>MSSTKQITLYTATFSPYAHRVRIALEEAGAEYTTYDVDILRNMPDWFPLVNPLKKIPAMTFGGPEVPPDQPSPESAKIAESLAMLEFIADLFPDAKLLPTDPVLRARARTFMALYENYVNGQFRDVWFLGTPADPLLQALEMLQGALPPDGGFAAGEWSIADAAVIPFLARMFPYLEAGLGLYS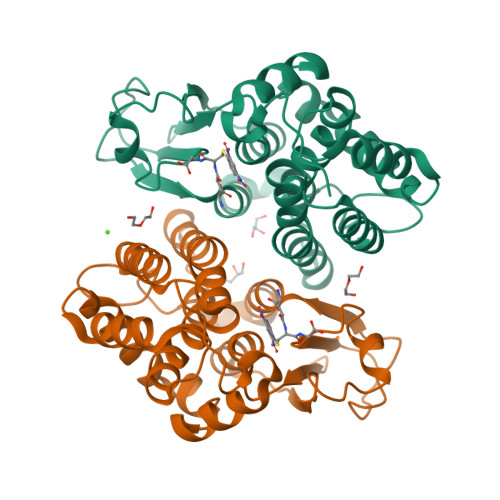KEDGVKMRKAMASERFARIRQYVRDCRARPSFANTWAGDAEQVEAAKTVPMLRVGEHHHHHH[2x]>MEAIAKYDFKATADDELSFKRGDILKVLNEECDQNWYKAELNGKDGFIPKNYIEMKPHPWFFGKIPRAKAEEMLSKQRHDGAFLIRESESAPGDFSLSVKFGNDVQHFKVLRDGAGKYFLWVVKFNSLNELVDYHRSTSVSRNQQI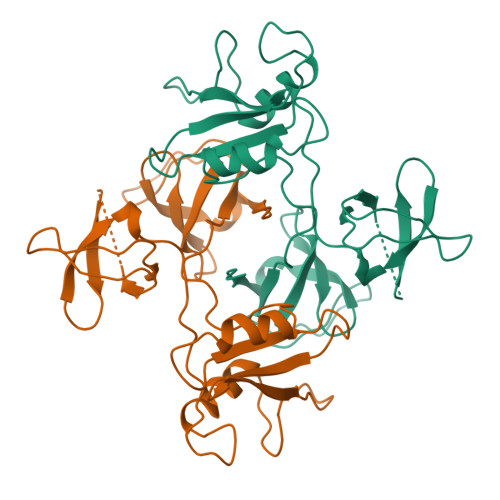FLRDIEQVPQQPTYVQALFDFDPQEDGELGFRRGDFIHVMDNSDPNWWKGACHGQTGMFPRNYVTPVNRNV[2x]> GPLGSMSQSNRELVVDFLSYKLSQKGYSWSQMAAVKQALREAGDEFELRYRRAFSDLTSQLHITPGTAYQSFEQVVNELFRDGVNWGRIVAFFSFGGALCVESVDKEMQVLVSRIA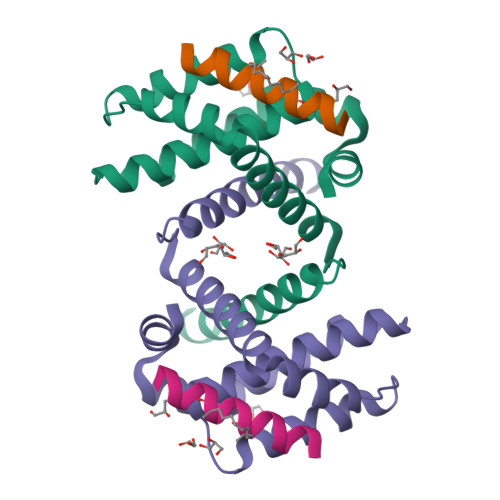AWMATYLNDHLEPWIQENGGWDTFVELYGNNAAAESRKGQER;> WIAQELRLIGDLFNAYYAX4-(5-aminopyrazin-2-yl)-1H-pyrrolo[2,3-b]pyridin-6-amine 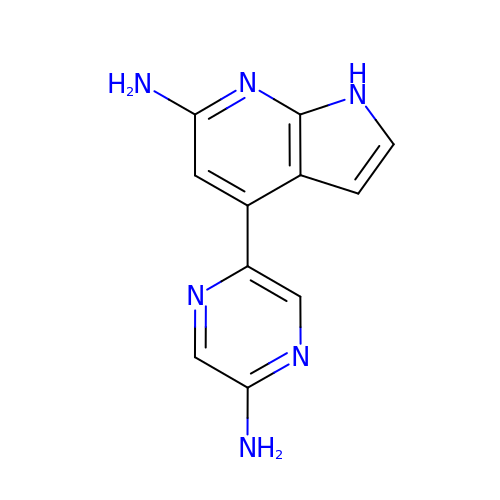| C11 H10 N6 | RYQGSVCSEHEBHC-UHFFFAOYSA-N> DGRGLSRAIPQNAEYTAECGSCHMAYPANLLPADKWRAITANLENHFGDNASLDPQVTARIEEYLVQHAAQNGKVMK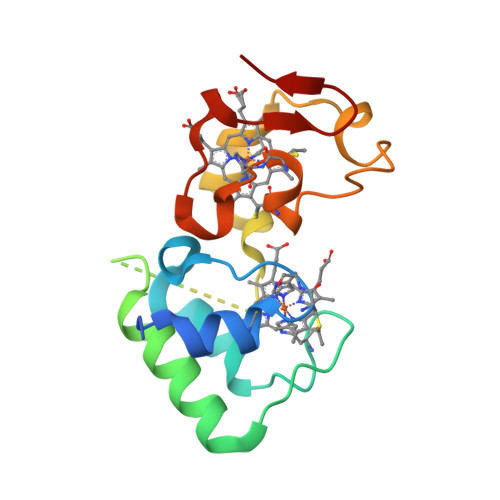NSTPLLAGAGPQKITEQAFFIRKHDEIPRRMVQDNPKVGSFSQCSNCHNLAEKGIFDEDTVNIPGFGRWDD>[2x]MAKDKEFQVLFVLTILTLISGTIFYSTVEGLRPIDALYFSVVTLTTVG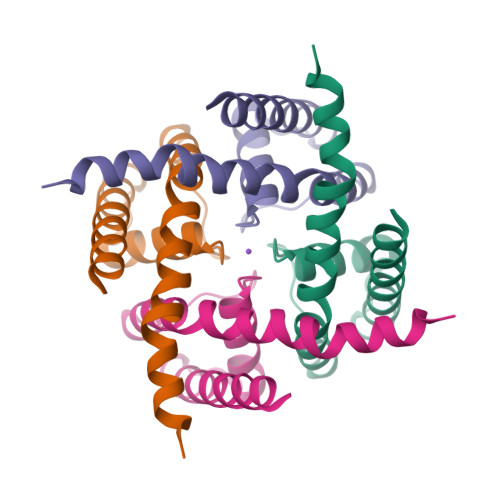DGDFSPQTDFGKIFTILYIFIGIGLVFGFIHKLAVNVQLPSILSNLVPR>VLPENMKRYMGRDAQRMNILAGRIIAETVRSTLGPKGMDKMLVDDLGDVVVTNDGVTILREMSVEHPAAKMLIEVAKTQEKEVGDGTTTAVVVAGELLRKAEELLDQNVHPTIVVKGYQAAAQKAQELLKTIACEVGAQDKEILTKIAMTSITGKGAEKAKEKLAEIIVEAVSAVVDDEGKVDKDLIKIEKKSGASIDDTELIKGVLVDKERVSAQMPKKVTDAKIALLNCAIEETASEMLKDMVAEIKASGANVLFCQKGIDDLAQHYLAKEGIVAARRVKKSDMEKLAKATGANVITNIKDLSAQDLGDAGLVEERKISGDSMIFVEECKHPKAVTMLIRGTTEHVIEEVARAVDDAVGVVGCTIEDGRIVSGGGSTEVELSMKLREYAEGISGREQLAVRAFADALEVIPRTLAENAGLDAIEILVKVRAAHASNGNKCAGLNVFTGAVEDMCENGVVEPLRVKTQAIQS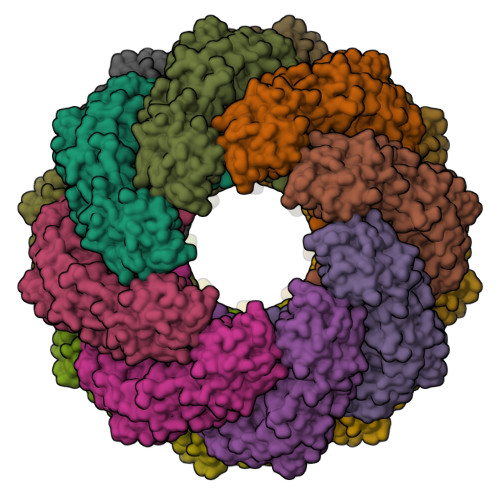AAESTEMLLRIDDVIAAE[16x]All ATAD2 orthologs share a characteristic N-terminal AAA ATPase domain and a C-terminal bromodomain. Additional functional studies allowed us to characterize the normal function of Atad2, and to show that it is a general auxiliary factor targeting acetylated histones and facilitating chromatin-templated processes by maintaining chromatin accessible. However, in contrast to FACT, Atad2 bears a bromodomain capable of specifically guiding the protein toward acetylated histones where it could act as a molecular motor thanks to its AAA ATPase domain. To elucidate the structural basis of the ATAD2–histone interaction, we co-crystallized the ATAD2 bromodomain with peptides derived from the acetylated H4 tail.

We previously found the preference of ATAD2 bromodomain for multiple acetylated histone tails, and we had observed that mouse Atad2 preferentially binds to H4K5ac. Consequently, we focussed on H4 acetylated on K5 and K12. Hence, the purified ATAD2 bromodomain was crystallized with H4 tail peptides monoacetylated at either of these two sites. As described for other bromodomains, water molecules occupy the bottom of the acetyl-lysine binding site. For the two acetylated H4 peptides, residues R3 to G7 and G9 to G13 are well resolved in the electron density maps (lower left). However, apart from these conserved interactions, which are also shared with the binding mode of the isolated acetyl-lysine residue, the binding mode of the H4K5ac- and H4K12ac-containing peptides outside the central binding pocket is highly diverse. In contrast, the interactions with H4K5ac were more optimal, containing a number of main-chain and side-chain hydrogen bonds, as well as a salt bridge interaction between H4R3 and D1066 (upper right).

> SMQEEDTFRELRIFLRNVTHRLAIDKRFRVFTKPVDPDEVPDYVTVIKQPMDLSSVISKIDLHKYLTVKDYLRDIDLICSNALEYNPDRDPGDRLIRHRACALRDTAYAIIKEELDEDFEQLCEEIQESR;> RGKGGKGLGKGGAY> AERSELTIHPKEFTTFVRNFNPFLGATNLHTTTDFIYEPLVVFNEMHGNTPVFRLAENFQMSDDLMSVTFDIRKGVKWSDGEAFTADDVVYSFNLVKEKPELDQSGINSWVTGVEKVNDYQVKFRLSEANSNVPYEIAKVPVVPKHVWSKVKDPSTFTNENPVGSGPFTVIDTFTPQLYIQCENPNYWDAANLDVDCLRVPQIANNDQFLGKVVNGEMDWTSSFVPDIDRTYAAASPKHHYWYPPAGTQAFVVNFKNPDAAKNEALTNVDFRRAFSMALDRQTIIDIAFYGGGTVNDFASGLGYAFEAWSDEKTHDKFKAYNSYNAEGAKKLLAKAGFKDVNKDGFVDTPSGKSFELLIQSPNGWTDFNNTVQLAVEQLAEVGIKARARTPDFSVYN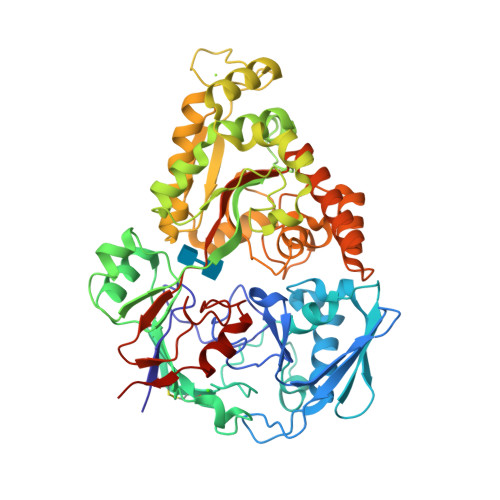QAMLEGTYDVAYTAYFHGADPYTYWNSAYNSALQSGDGMPRFAMHFYKNEKLDGLLNSFYKTADKQEQLEIAHGIQQIIAQDQVTIPVLSGAYMYQYNTTRFTGWWNEENPKGRPNIWAGIPERLLHVLDLKPVKHHHHHH> MTNELINGVALADTPEKLVKAVQELALAKDVAAIPTLIAVFGYNNPTAAAIASTALVQLGEVAVPQLLTQIDDYNYGARAYSIRTLAAIADPRALDVLIDAAATDFAPSVRRAAAKGLGNLHWHKLEFPDNQTAPKKALETLLFISQDAEWS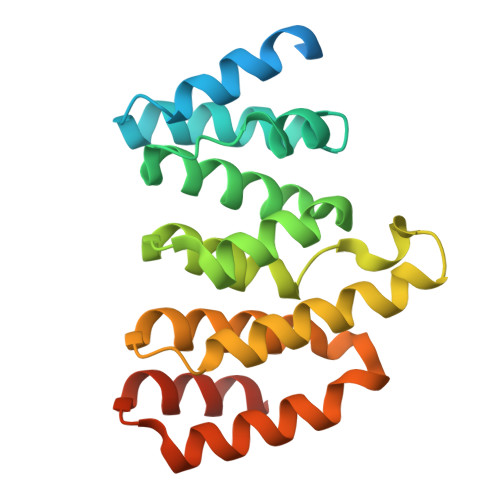IRYAAIVGLQGLVNIPDLQQPIHTRLKEMLASDAEKAVRARILLAQSQLEHHHHHH N-(acetylcarbamoyl)-beta-D-glucopyranosylamine | C9 H16 N2 O7 | 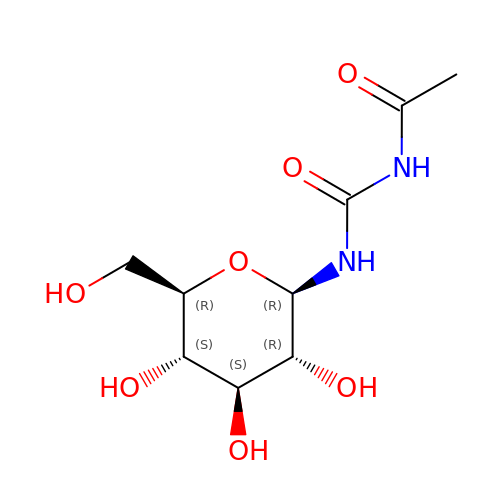UQKBNLXZEGBQAF-JAJWTYFOSA-N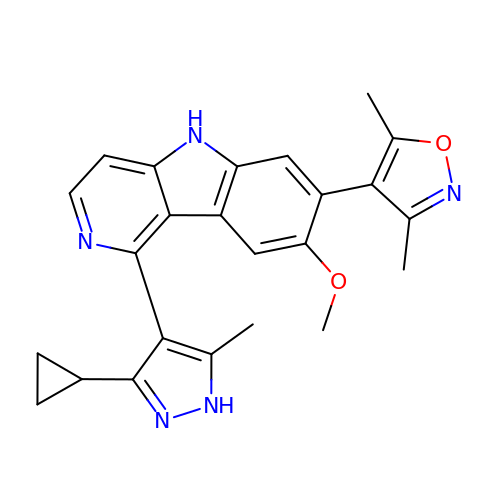1-(3-cyclopropyl-5-methyl-1H-pyrazol-4-yl)-7-(3,5-dimethyl-1,2-oxazol-4-yl)-8-methoxy-5H-pyrido[4,3-b]indole | C24 H23 N5 O2 | WHDUHJYPRJXLGF-UHFFFAOYSA-N>[4x]MHHHHHHNNDNNTILGFDVNLICDFFLNTERQGPGSPEVTLKALSFIDNLTNKSLIAD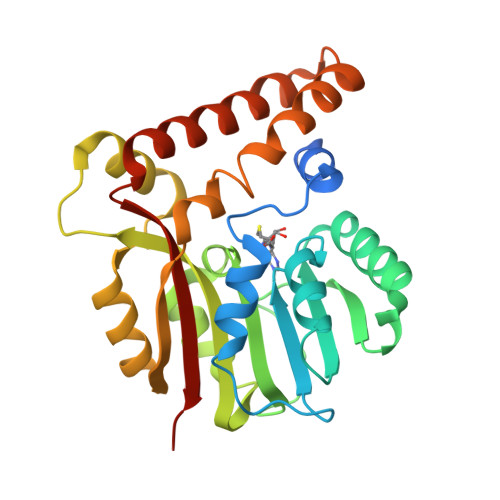LGCGTGGQTMILAQHVPGKITGIDFFPGFIERFNKNAEKLNLQNRVKGIVGSMDDLSFEKDSLDLIWSEGAIYNIGFERGLKEWRNYLKPGGYLAVSESVWFTDQRPAEIHDFWMSAYTEIDTVPNKVAQIQKAGYIPVATFILPENCWIEHYFAPQAKAEEIFRRKHAGSRIVEELITSNHHEAELYSKYKAYYGYAFFICKKGFSLRR6-[(cyclopropanecarbonyl)amino]-4-{[2-methoxy-3-(pyrimidin-2-yl)phenyl]amino}-N-methylpyridazine-3-carboxamide 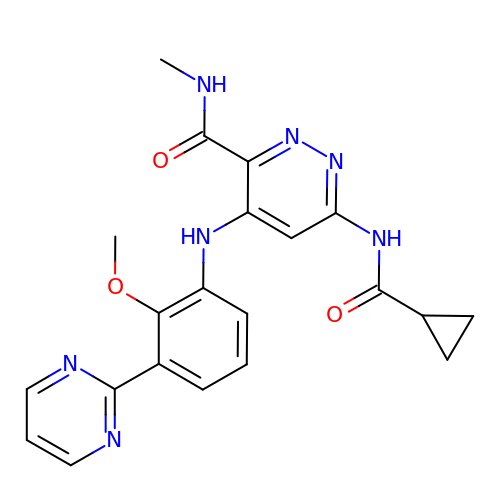| C21 H21 N7 O3 | XPHMHCUYKWFASJ-UHFFFAOYSA-N> GAMGSMDTQAGSV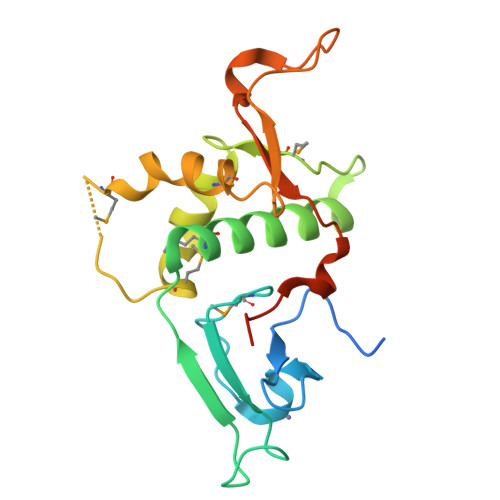DEENGRQLGEVELQCGICTKWFTADTFGIDTSSCLPFMTNYSFHCNVCHHSGNTYFLRKQANLKEMCLSALANLTWQSRTQDEHPKTMFSKDKDIIPFIDKYWECMTTRQRPGKMTWPNNIVKTMSKERDVFLVKEHPDPGSKDPEEDYPKFGLLDQDLSNIGPAYDNQKQSSAVSTS> MKPITFVVLASVMKELSLKASPLRSETAEGIVVVTTWIEKILTDLKVQHKRVPCGKEEVSLFLTAIENSWIHLRRKKRERVRQLREVPRAPEDVIQALEEKKGVAGQYLFKCLINVKKEVDDALVEMHWVEGQNRDLMNQLCTYIRNQIFRLVAVNLEHHHHH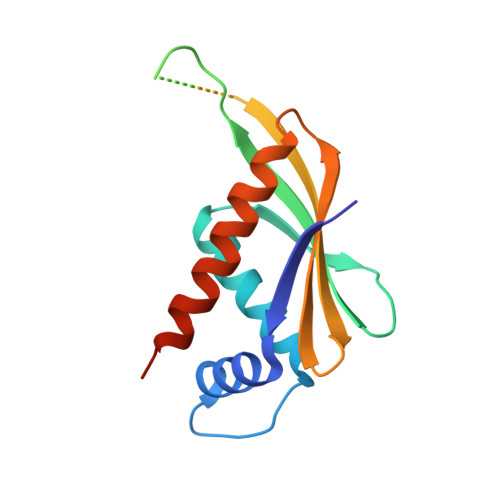H>MKITAVEPFILHLPLTSESISDSTHSITHWGVVGAKITTSDGIEGYGFTGTHAHLPSDRLITSCIS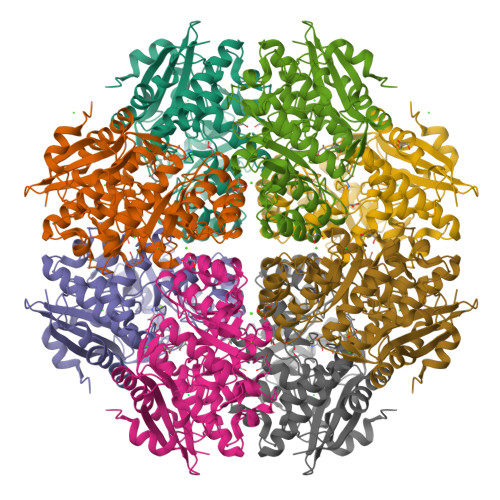DCYAPLLLGEDASDHSRLWTKLARYPSLQWVGRAGITHLALAAVDVALWDIKAKKAGVPLWHYLGGARTAGVEAYNTDIGWLSFTLEDLLAGSARAVEEDGFTRLKIKVGHDDPNIDIARLTAVRERVDSAVRIAIDGNGKWDLPTCQRFCAAAKDLDIYWFEEPLWYDDVTSHARLARNTSIPIALGEQLYTVDAFRSFIDAGAVAYVQPDVTRLGGITEYIQVADLALAHRLPVVPHAGEMSQVHVHLSYWHPASTILEYIPWIKDHFEEPIHVRDGVYKRPEQPGASTTPLAESFTRYGKAVK[16x]>MHHHHHHENLYFQADQTNPYKLMDEAAQKTFDRLKNEQPQIRANPDYLRTIVDQELLPYVQVKYAGALVLGQYYKSATPAQREAYFAAFREYLKQAYGQALAMYHGQTYQIAPEQPLGDKTIVPIRVTIIDP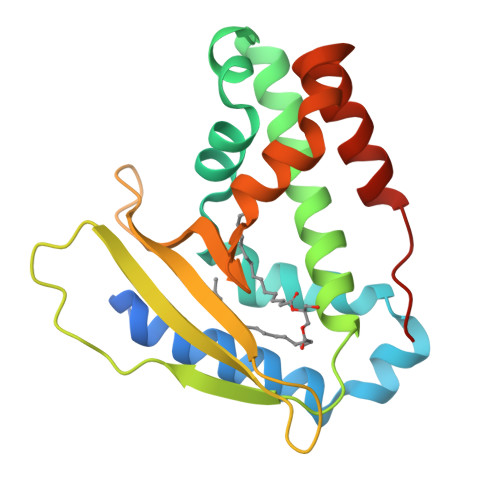NGRPPVRLDFQWRKNSQTGNWQAYDMIAEGVSMITTKQNEWGTLLRTKGIDGLTAQLKSISQQKITLEEKK[2x]>[2x]MKVL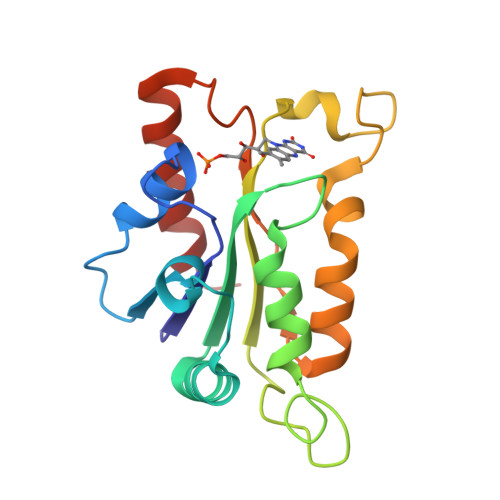VLAFHPNMEQSVVNRAFADTLKDAPGITLRDLYQEYPDEAIDVEKEQKLCEEHDRIVFQFPLYWYSSPPLLKKWLDHVLLYGWAYGTNGTALRGKEFMVAVSAGAPEEAYQAGGSNHYAISELLRPFQATSNFIGTTYLPPYVFYQAGTAGKSELAEGATQYREHVLKSF>[2x]MAKPLTDQEKRRQISIRGIVGVENVAELKKSFNRHLHFTLVKDRNVATTRDYYFALAHTVRDHLVGRWIRTQQHYYDKCPKRVYYLSLEFYMGRTLQNTMINLGLQNACDEAIYQLGLDIEELEEIEEDAGLGNGGLGRLAACFLDSMATLGLAAYGYGIRYEYGIFNQKIRDGWQVEEADDWLRYGNPWEKSRPEFMLPVHFYGKVEHTNTGTKWIDTQVVLALPYDTPVPGYMNNTVNTMR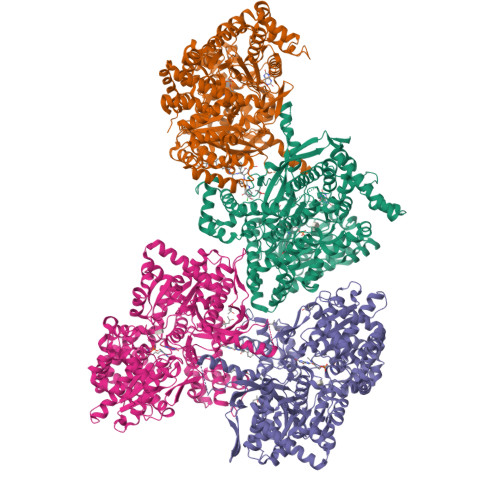LWSARAPNDFNLRDFNVGDYIQAVLDRNLAENISRVLYPNDNFFEGKELRLKQEYFVVAATLQDIIRRFKASKFGSTRGAGTVFDAFPDQVAIQLNDTHPALAIPELMRIFVDIEKLPWSKAWELTQKTFAYTNHTVLPEALERWPVDLVEKLLPRHLEIIYEINQKHLDRIVALFPKDVDRLRRMSLIEEEGSKRINMAHLCIVGSHAVNGVAKIHSDIVKTKVFKDFSELEPDKFQNKTNGITPRRWLLLCNPGLAELIAEKIGEDYVKDLSQLTKLHSFLGDDVFLRELAKVKQENKLKFSQFLETEYKVKINPSSMFDVQVKRIHEYKRQLLNCLHVITMYNRIKKDPKKLFVPRTVIIGGKAAPGYHMAKMIIKLITSVADVVNNDPMVGSKLKVIFLENYRVSLAEKVIPATDLSEQISTAGTEASGTGNMKFMLNGALTIGTMDGANVEMAEEAGEENLFIFGMRIDDVAALDKKGYEAKEYYEALPELKLVIDQIDNGFFSPKQPDLFKDIINMLFYHDRFKVFADYEAYVKCQDKVSQLYMNPKAWNTMVLKNIAASGKFSSDRTIKEYAQNIWNVEPSDLKISLSNESNKVNGN>[2x]MSMSTSTEVIAHHWAFAIFLIVAIGLCCLMLVGGWFLGGRARARSKNVPFESGIDSVGSARLRLSAKFYLVAMFFVIFDVEALYLFAWSTSIRESGWVGFVEAAIFIFVLLAGLVYLVRIGALDWTPARSRRERMNPETNSIANRQR;>MNMLALTIILPLIGFVLLAFSRGRWSENVSAIVGVGSVGLAALVTAFIGVDFFANGEQTYSQPLWTWMSVGDFNIGFNLVLDGLSLTMLSVVTGVGFLIHMYASWYMRGEEGYSRFFAYTNLFIASMVVLVLADNLLLMYLGWEGVGLCSYLLIGFYYTDPKNGAAAMKAFVVTRVGDVFLAFALFILYNELGTLNFREMVELAPAHFADGNNMLMWATLMLLGGAVGKSAQLPLQTWLADAMAGPTPVSALIHAATMVTAGVYLIARTHGLFLMTPEVLHLVGIVGAVTLLLAGFAALVQTDIKRVLAYSTMSQIGYMFLALGVQAWDAAIFHLMTHAFFKALLFLASGSVILACHHEQNIFKMGGLRKSIPLVYLCFLVGGAALSALPLVTAGFFSKDEILAGAMANGHINLMVAGLVGAFMTSLYTFRMIFIVFHGKEQIHAHAVKGVTHSLPLIVLLILSTFVGALIVPPLQGVLPQTTELAHGSMLTLEITSGVVAVVGILLAAWLWLGKRTLVTSIANSAPGRLLSTWWYNAWGFDWLYDKVFVKPFLGIAWLLKRDPLNSMMNIPAVLSRFAGKGLLLSENGYLRWYVASMSIGAVVVLALLMVLR[2x];>MLLPWLILIPFIGGFLCWQTERFGVKVPRW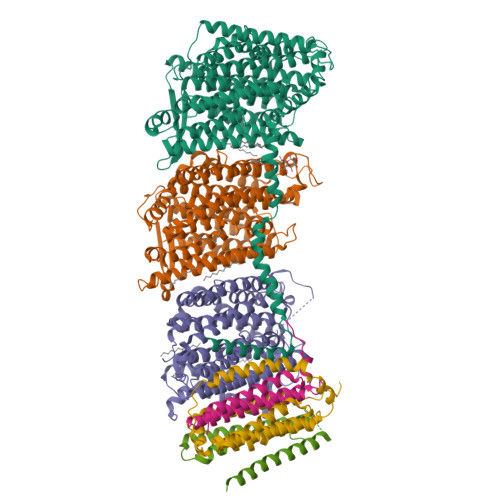IALITMGLTLALSLQLWLQGGYSLTQSAGIPQWQSEFDMPWIPRFGISIHLAIDGLSLLMVVLTGLLGVLAVLCSWKEIEKYQGFFHLNLMWILGGVIGVFLAIDMFLFFFFWEMMLVPMYFLIALWGHKASDGKTRITAATKFFIYTQASGLVMLIAILALVFVHYNATGVWTFNYEELLNTPMSSGVEYLLMLGFFIAFAVKMPVVPLHGWLPDAHSQAPTAGSVDLAGILLKTAAYGLLRFSLPLFPNASAEFAPIAMWLGVIGIFYGAWMAFAQTDIKRLIAYTSVSHMGFVLIAIYTGSQLAYQGAVIQMIAHGLSAAGLFILCGQLYERIHTRDMRMMGGLWSKMKWLPALSLFFAVATLGMPGTGNFVGEFMILFGSFQVVPVITVISTFGLVFASVYSLAMLHRAYFGKAKSQIASQELPGMSLRELFMILLLVVLLVLLGFYPQPILDTSHSAIGNIQQWFVNSVTTTRP[2x];>[2x]MTITPQNLIALLPLLIVGLTVVVVMLSIAWRRNHFLNATLSVIGLNAALVSLWFVGQAGAMDVTPLMRVDGFAMLYTGLVLLASLATCTFAYPWLEGYNDNKDEFYLLVLIAALGGILLANANHLASLFLGIELISLPLFGLVGYAFRQKRSLEASIKYTILSAAASSFLLFGMALVYAQSGDLSFVALGKNLGDGMLNEPLLLAGFGLMIVGLGFKLSLVPFHLWTPDVYQGAPAPVSTFLATASKIAIFGVVMRLFLYAPVGDSEAIRVVLAIIAFASIIFGNLMALSQTNIKRLLGYSSISHLGYLLVALIALQTGEMSMEAVGVYLAGYLFSSLGAFGVVSLMSSPYRGPDADSLFSYRGLFWHRPILAAVMTVMMLSLAGIPMTLGFIGKFYVLAVGVQAHLWWLVGAVVVGSAIGLYYYLRVAVSLYLHAPEQPGRDAPSNWQYSAGGIVVLISALLVLVLGVWPQPLISIVRLAMPLM;>[2x]MEFAFYICGLIAILATLRVITHTNPVHALLYLIISLLAISGVFFSLGAYFAGALEIIVYAGAIMVLFVFVVMMLNLGGSEIEQERQWLKPQVWIGPAILSAIMLVVIVYAILGVNDQGIDGTPISAKAVGITLFGPYVLAVELASMLLLAGLVVAFHVGREERAGEVLSNRKDDSAKRKTEEHA;>[2x]MIPLQHGLILAAILFVLGLTGLVIRRNLLFMLIGLEIMINASALAFVVAGSYWGQTDGQVMYILAISLAAAEASIGLALLLQLHRRRQNLNIDSVSEMRG> NEAIECHLSDLLQQLTSVNASKPSERGLVRQEEAEDPACIPIFWVSKWVDYSDKYGLGYQLCDNSVGVLFNDSTRLILYNDGDSLQYIERDGTESYLTVSSHPNSLMKKITLLNYFRNYMSEHLLKAGANITPREGDELARLPYLRTWFRTRSAIILHLSNGTVQINFFQDHTKLILCPLMAAVTY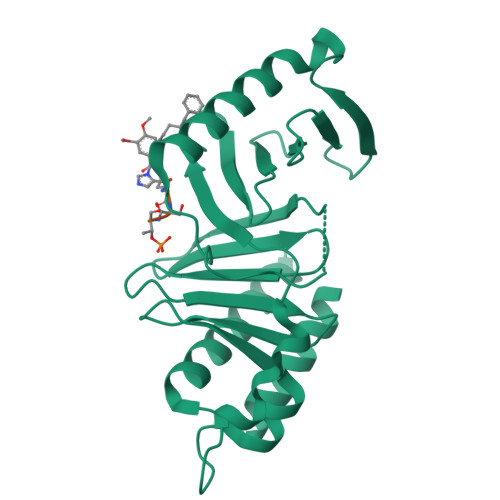INEKRDFQTYRLSLLEEYGCCKELASRLRYARTMVDKLLSSRSASNRLKAS During an analysis of Acinetobacter baumannii strain AB 5075 genome we have identified an open reading frame (ORF) encoding a protein with the proposed muramidase activity that structurally resembles bacteriophage endolysins. This enzyme carries a C-terminal domain with predicted α-helical organization and a pronounced localized positive charge. Conservative domain (aa 40–177) is typical for phage endolysins and bacterial autolysins, and usually degrades peptidoglycan by a N-acetyl-β-d-muramidase activity utilizing a Glu-Asp-Thr catalytic triad. AcLys, one of such “naturally artilyzed” protein with the C-terminal α-helical domain demonstrates moderate activity against viable Gram-negative bacteria from outside.

The crystal structure of AcLys was refined to 1.2 Å resolution. There is one protein monomer is the asymmetric unit. The final model comprises one subunit of the protein (149 residues), 229 water molecules as well as sulfate and glycerol molecules. The first 47 N-terminal residues were not observed in electron density maps apparently due to high mobility of these residues or to limited proteolysis. The protein has overall α-helical architecture typical for lysozyme family, and is composed of seven α-helices: α2: residues 54–64, α3: 101–122, α4: 129–142, α5: 144–149, α6: 151–157, α7: 161–170 and α8: 180–193. Active site is formed by conserved catalytic triad: Glu64, Asp73 and Thr79 are clearly seen in the electron density. Glu64 forms salt bridge to conserved Arg185 which lies on the C-terminal helix α8. This salt bridge is a well-known feature of the known endolysins of P21 and P22 families. In case of AcLys the loop harbors an increased number of positively charged residues, including conserved Arg185, Arg186, Arg190 and Lys180 (also found in case of DLP12 endolysin from E. coli), unique Arg184—which is a part of positively charged patch consisting of three arginines, as well as Lys195 and Lys196. These residues surround the loop forming positive charge on their surface and thus could potentially bind and penetrate the cell membrane.

> MHHHHHHENLYFQSTKPFFDAARVIAGGKLTQAQVDDLNKVVEKLAPGGKTTSDDGIDLITSFEGTRFNAYDDGVGVWTIGTGTTVYPNGVKVKKGDTCTAEQAKTYFKHDLAKFEKTVNESVTAPLTQNQFDALVSLTYNIGSGAFNNSTLLKKLNKGDYQGAADQFLVWNKAGGKVMKGLVRRREAERALFLKK>SNAGKNVMVEPHRHEGVFICRGKEDALVTKNLVPGESVYGEKRVSISEGDDKIEYRAWNPFRSKLAAAILGGVDQIHIKPGAKVLYLGAASGTTVSHVSDIVGPDGLVYAVEFSHRSGRDLINLAKKRTNIIPVIEDARHPHKYRMLIAMVDVIF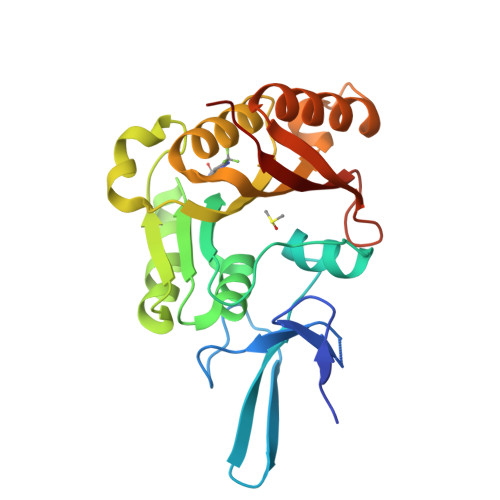ADVAQPDQTRIVALNAHTFLRNGGHFVISIKANCIDSTASAEAVFASEVKKMQQENMKPQEQLTLEPYERDHAVVVGVYRPPPKVKN[2x]>[2x]GPLGSARRLYVGNIPFGITEEAMMDFFNAQMRLG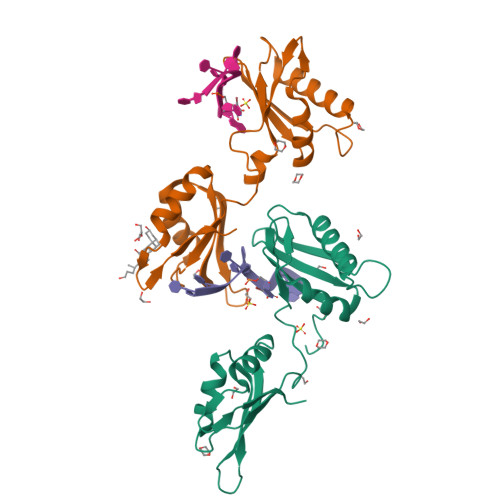GLTQAPGNPVLAVQINQDKNFAFLEFRSVDETTQAMAFDGIIFQGQSLKIRRPHDYQPLPGAHKLFIGGLPNYLNDDQVKELLTSFGPLKAFNLVKDSATGLSKGYAFCEYVDINVTDQAIAGLNGMQLGDKKLLVQRAS>PPGPPGPPGEKGSPGAQGPPGPP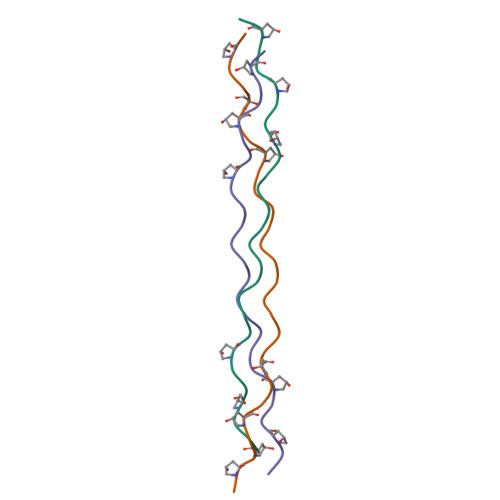GPPG[3x]>[4x]GSMSEQSICQARAAVMVYDDANKKWVPAGGSTGFSRVHIYHHTGNNTFRVVG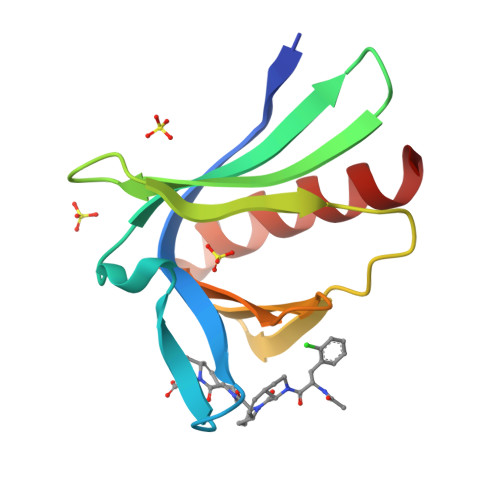RKIQDHQVVINCAIPKGLKYNQATQTFHQWRDARQVYGLNFGSKEDANVFASAMMHALEVL2-(1,1-DIFLUOROETHOXY)-1,1,1-TRIFLUOROETHANE | C4 H5 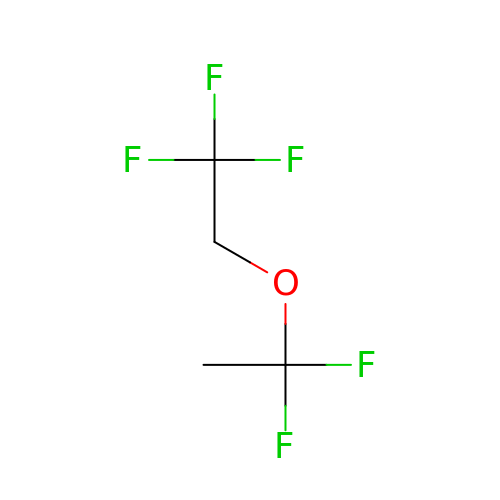F5 O | LUGFHDZVRRASHY-UHFFFAOYSA-N>[2x]SKNKEDKRNAEYRLAFEQLNFVGADSKTPILKSFIEDKGTRIDEITFESMIPIETWKSYIPQLQTSLNISIISIEQGASKRIVIIKSMAGDAKIPKYLPWDDKYIEEQEGVVVVGQTFSGNIKIDLNKSPHILSAGETGSGKSVILRCILWQLLKQGAIAYMVDFKGGVEFGLEYEKVGQV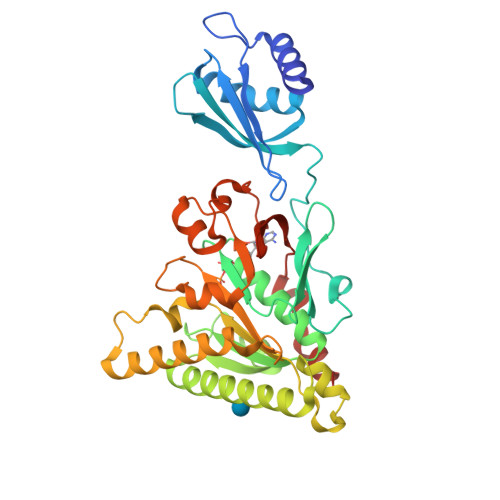ITEVDAAEKLFKYLVDENAKRLKLLRESGSKNIGEYNKKFEGEELKRIIVVIDELAELMDKTGVDDETRAKLVRIEGYTSTLARLSRATGINLCIGVQRPDAKVITGQIKNNVPVRICGRFADSKASEIVLSNTKAKDLPEVKGRFLFKLGADTVQFQAFYFDDDKHFIPNKILKLRK> SMIVRGINMTKIKLESPGFMVHKKLKSMSQSYGVMMTGVPAEVLG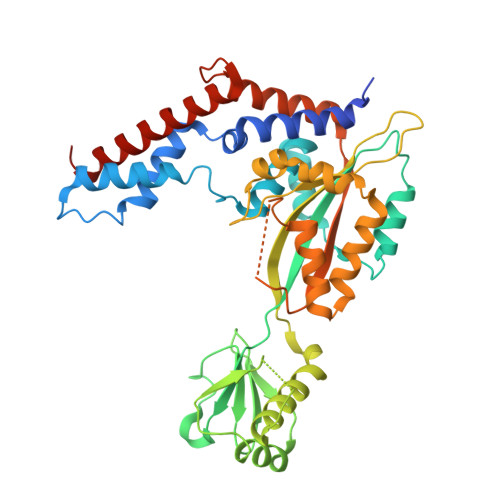QMQAERSIPSINKTGNLKQQIAKEVSKVCHMMTEPTQSCGQASNDVCELLLGKIEAEKFHFTKYEALSADGDNLKNVLENTAPSSTNLLIRFEIDREDPPIVLVKTKNENFNPETAVKNKIYLLENKLYFIDKMGNLFNLGPGKKKCTQLFNAIGDSAEYSLCDPFVLEEPEKPEDFAISEIVDIFNEQKERFDFWIGSHSFTIYIPQTLGESPRQFYPYQAYFGSHTLQDWFVSDKDEYLSRIGIDKYIEKLAVLGKTTNTKERSDIYAEFFSKRGREAFFCAHLNEKRQPLRVKFKITEINPELALKNLQETQEFIDTHPGENPSDKVENYRNRAKLAMTEHLESLLDIKPESS> MTENTKNENITNILTQKLIDTRTVLIYGEINQELAEDVSKQLLLLESISNDPITIFINSQGGHVEAGDTIHDMIKFIKPTVKVVGTGWVAAAGITIYLAAEKENRFSLPNTRYMIHQPAGGVQGQSTEIEIEAKEIIRMRERINRLIAEATGQSYEQISKDTDRNFWLSV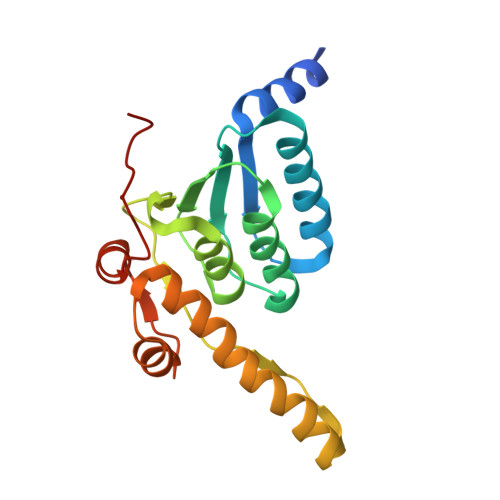NEAKDYGIVNEIIENRDGLK>[2x]SNAM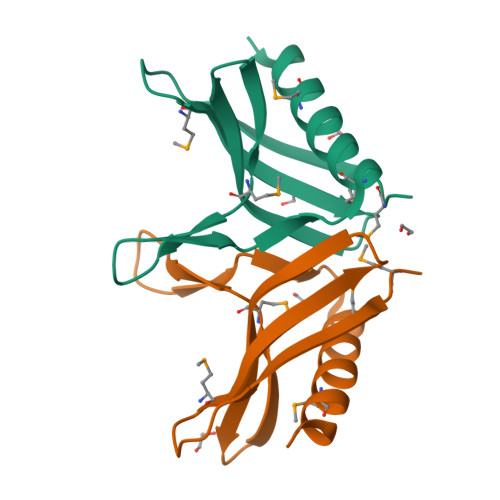KVTDVRLRKIQTDGRMKALVSITLDEAFVIHDLRVIEGNSGLFVAMPSKRTPDGEFRDIAHPINSDMRQEIQDAVMKVYDETD> SMTIQEIIQQRNIRSLFHFTHSDNLTSILDNGLMSRSELDNENNEYNCNDEERIDGHPDAICLSVSYPNAKMFYKYRCLKPGDWVILEINPSVLWAKDCAFYPTNAASNNVRFINLDLMKGAEAFSALFSENVFGIQRDVNLPSEYTTDVQAAILVFEKIPPSYIISTFHPNKESAEHFKRLYPQTIQRYYDNLNARTLYSQRHYYLG

Modification of nucleic acids by ADP-ribosylation is catalyzed by various ADP-ribosyltransferases, including the DarT enzyme. The latter is part of the bacterial toxin-antitoxin (TA) system DarTG, which was shown to provide control of DNA replication and bacterial growth as well as protection against bacteriophages. Using structural and biochemical approaches, we show that DarT1-NADAR is a TA system for reversible ADP-ribosylation of guanosine bases. DarT1 evolved the ability to link ADP-ribose to the guanine amino group, which is specifically hydrolyzed by NADAR.

To confirm and characterize DarT1-catalyzed guanine ADP-ribosylation, we determined the structures of full-length E. coli C7 DarT1E152A in its pre- and post-reaction states. Co-crystallization of E. coli C7 DarT1E152A with NAD+ as well as with carba-NAD+, a non-hydrolyzable NAD+ analog, and an ssDNA 5-mer allowed insights into the substrate-bound state of DarT1, while co-crystallization with NAD+ and the ssDNA 5-mer gave a structure at 1.63 Å of the product-bound state. (I) Overlay of the crystal structures of E. coli C7 DarT1E152A in complex with NAD+ and carba-NAD+:DNA to represent the pre-reaction, i.e., NAD+:DNA-bound state. The distal-ribose C1 linkage to the base and the potential proton transfer from the guanine N2 onto D54 and R52 over the water molecule w88 involved in the mechanism is indicated with black arrows. The interplay of key residues in the active site for catalyzing the reaction is enabled by their proximity, allowing coordination of the guanosine, the NAM moiety, and the distal ribose, which promote NAD+ polarization, NAM-ribose bond cleavage, and generation of an oxocarbenium ion intermediate. Of particular note is that comparison of DarT1 in the carba-NAD+:DNA-bound state with the ADPr-DNA-bound state revealed that the side-chain flexibility of R51 in DarT2 could not be observed in DarT1. The corresponding arginine residue in DarT1 (R52) hydrogen bonds in all captured states to the β-phosphate and is furthermore ideally hydrogen-bonded by D54, indicating their interplay for catalysis.> RP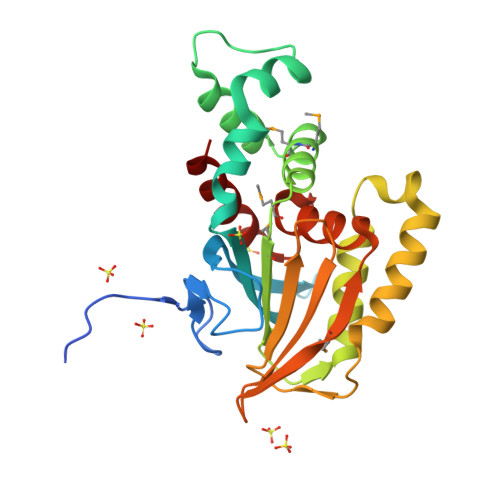VQNDDKTDAFPSHTESIQVDSSVSDFPLTITALNFPVSTTFKLLGYGQAHVTFLRFKVYALGLYLAENDENLVSDTLNETYLHKYFLDVDDSKTPKENLARLLKRDDSKSVMMIDDLLDSGMRMLAKITPVRNTDFKHLKEGLVKTISKHPDVANNKDTLAKGLSELNDAFSRKGSVRKNDDLIIELLANGALQFSYHDSKNNEFEVMGVVNNQLVGKFLFSQYLCGEKSPSPQAKKTAIDKLITLL> LKESPSGYLRSGEGDTGCGELVWVGEPLTLRTAETITGKYGVWMRDPKPTYPYTQETTWRIDTVGTDVRQVFEYDLISQFMQGYPSKVHILPRPLESTGAVVYSGSLYFQGAESRTVIRYELNTETVKAEKEIPGAGYHGQFPYSWGGYTDIDLAVDEAGLWVIYSTDEAKGAIVLSKLNPENLELEQTWETNIRKQSVANAFIICGTLYTVSSYTSADATVNFAYDTGTGISKTLTIPFKNRYKYSSMIDYNPLEKKLFAWDNLNMVTYDIRLSKM

Inherited missense mutations in the myocilin (MYOC) gene, within its olfactomedin (OLF) domain, constitute the strongest genetic link to primary open-angle glaucoma via a toxic gain of function, and thus MYOC is an attractive precision-medicine target. Myocilin has no known function, and there is no glaucoma phenotype in Myoc knockout mice or in individuals with a homozygous N-terminal truncation mutation or hemizygous deletion of MYOC, but rare non-synonymous coding mutations lead to toxic intracellular sequestration of misfolded myocilin. However, not all mutations in MYOC cause glaucoma, and common variants are expected to be neutral polymorphisms. Among the common features associated with pathogenic myocilin misfolding, we demonstrate that a single metric, OLF thermal stability, can robustly segregate benign from early-onset disease variants.

At the outset of our study, five variants could be confidently predicted as benign polymorphisms: T293K, T353I, K398R, A445V and K500R. These mutations are all found on the protein surface and well documented in the literature. Three of these variants harbor conservative substitutions (Lys to Arg, Ala to Val). Assessment of spent media from cells expressing each of the 16 full-length myocilin variants revealed WT-like secretion for T256M, R296H, L303I, S313F, V329M, S331L, T353I, A445V, V449I and K500R. Structural integrity was further confirmed by high-resolution crystal structures, which were solved for 11 OLF variants. No gross changes from WT OLF were detected for the structures of T293K, R296H, L303I, V329M, S331L, E352K, T353I, K398R, A445V, V449I or K500R, indicating that these mutations are accommodated within the native five-bladed β-propeller fold and do not perturb the dinuclear calcium-containing site.> MGSDKIHHHHHHMVRLSEAEVQNPKLGEYQCLADLNLFDSPECTRLATQSASGRHLWVTSNHQNLAVEVYLCEDDYPGWLSLSDFDSLQPATVPYQAATFSESEIKKLLAEVIAFTQKAMQQSNYYLWGGTVGPNYDCSGLMQAAFASVGIWLPRDAYQQEGFTQPITIAELVAGDLVFFGTSQKATHVGLYLADGYYIHSSGKDQGRDGIGIDILSEQGDAVSL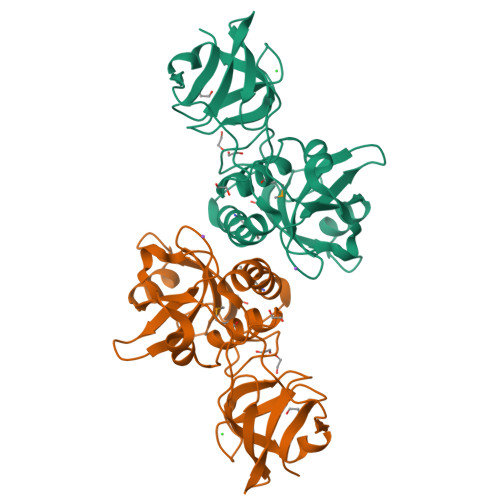SYYQQLRGAGRVFKSYEPQRR>[2x]AMKDLKGTKTAENLKQGFIGESMANRRYLYFAKRADEEGYPEIAGLLRSIAEGETAHAFGHLDFIRQGGLTDPATDKPIGTLEQMIESAIAGETYEWTQMYPGFAKVAREEGFPEVAEWFETLARAEKSHAEKFQNVLKQLKGGT

One such protein is sulerythrin (SulE), a ruberythrin-like protein isolated from the thermophilic archeon Sulfolobus tokodaii. SulE lacks the characteristic C-terminal, rubredoxin-like FeS4 domain of ruberythrins and contains a binuclear metal centre that coordinates iron and zinc when isolated from S. tokodaii. In contrast to other members of the ruberythrin family, a crystal structure of native SulE shows that it forms homodimers through domain swapping, with each monomer contributing two α-helices to give two four-helix bundles that each harbour a solvent-accessible, single dimetal site. The exact function of SulE is unknown, but it is presumed to be involved in reactions against oxidative stress.

In order to test the effect of the total absorbed dose on SpReAD analysis, data collection at higher flux values was repeated on the same crystal used at 5% beamline flux, choosing distinct, non-overlapping positions at least 50 µm apart. Data sets at 13.5 keV and nine energies over the rising Fe K edge were collected at 10% and 100% flux. Using RADDOSE-3D, the total average diffraction-weighted dose was calculated to be 0.26 MGy for 5% flux, 0.52 MGy for 10% flux and 2.70 MGy for 100% flux. The SpReAD analysis was then repeated for the data collected at 10% and 100% beamline flux, refining the f′′ contribution for each of the two Fe-2 and Fe-4 positions observed at 100% flux separately. While there was no difference in the oxidation states of all iron ions between 5% and 10% flux, at 100% flux a clear difference was visible for Fe-2 and Fe-4 at position 2, where the edge position was coincident with Fe-1 and Fe-3, suggesting that iron ions at this position are reduced.>[4x]MGHHHHHHHHHHSSGHIEGRHMQFEVLKRFFPKESLKNCKGALWVHTASIGEFNTFLPILKELKREHRILLTYFSPRAREYLKTKSDFYDCLHPLPLDNPFSVKRFEELSKPKALIVVEREFWPSLII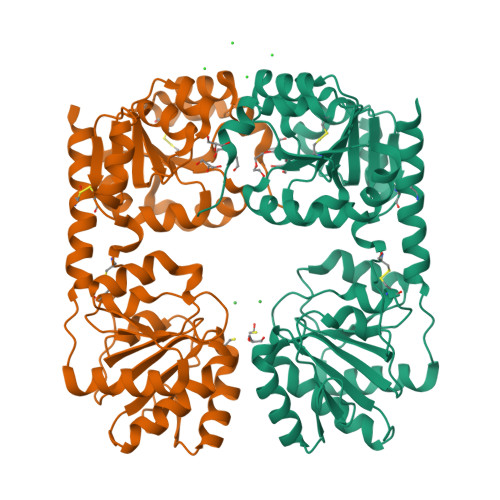FTKVPKILVNAYAKGSLIEKILSKKFDLIIMRTQEDVEKFKTFGAKRVFSCGNLKFICQKGKGIKLKGEFIVAGSIHTGEVEIILKAFKEIKKTYSSLKLILVPRHIENAKIFEKKARDFGFKTSFFENLEGDVILVDRFGILKELYPVGKIAIVGGTFVNIGGHNLLEPTCWGIPVIYGPYTHKVNDLKEFLEKEGAGFEVKNETELVTKLTELLSVKKEIKVEEKSREIKGCYLEKLREFLRGL> MALEGLRKKYKTRQELVKALTPKRRSIHLNSNGHSNGTPCSNADVLAHIKHFLSLAANSLEQHQQPISIVFQNKKKKGDTNSPDIHTTLDFPLNGPHLSTHQFKLKRCAILLNLLKVVMEKLPLGKNTTVRDIFYSNVELFQRQANVVQWLDVIRFNFKLSPRKSLNIIPAQKGLVYSPFPIDIYDNILTCENEPKMQKQTIFSGKPCLIPFFQDDAVIKLGTTSMCNIVIVEKEAVFTKLVNNYHKLSTNTMLITGKGFPDFLTRLFLKKLEQYCSNLISDCSIFTDADPYGISIALNYTHSNERNAYICTMANYKGIRITQVLAQNNEVHNKSIQLLSLNQRDYSLAKNLIASLTANSWDIATSPLKNVVIECQREIFFQKKAEMNEIDAGIFKYKSRHHHHHHHHHHGDYKDDDDKDYKDDDDKDYKDDDDK;> MARDITFLTVFLESCGAVNNDEAGKLLSAWTSTVRIEGPEPTDSNSLYIPLLPPGMLKIKLNFKMNDRLVTEEQELFTKLREIVGSSIRFWEEQLFYQVQDVSTIENHVILSLKCTILTDAQISTFISKPRELHTHAKGYPEIYYLSELSTTVNFFSKEGNYVEISHVIPHFNEYFSSLIVSQLEFEYPMVFSMISRLRLKWQQSSLAPISYALTSNSVLLPIMLNMIAQDKSSTTAYQILCRRRGPPIQNFQIFSIPAVTYNK;> MSKVFIATANAGKAHDADIFSVSACNSFTVSCSGDGYLKVWDNKLLDNENPKDKSYSHFVHKSGLHHVDVLQTIERDAFELCLVATTSFSGDLLFYRITREDETKKVIFEKLDLLDSDMKKHSFWALKWGASNDRLLSHRLVATDVKGTTYIWKFHPFADESNSLTLNWSPTLELQGTVESPMTPSQFATSVDISERGLIATGFNNGTVQISELSTLRPLYNFESQHSMINNSNSIRSVKFSPQGSLLAIAHDSNSFGCITLYETEFGERIGSLSVPTHSSQASLGEFAHSSWVMSLSFNDSGETLCSAGWDGKLRFWDVKTKERITTLNMHCDDIEIEEDILAVDEHGDSLAEPGVFDVKFLKKGWRSGMGADLNESLCCVCLDRSIRWFREAGGK;> MSIEEEDTNKITCTQDFLHQYFVTERVSIQFGLNNKTVKRINKDEFDKAVNCIMSWTNYPKPGLKRTASTYLLSNSFKKSATVSLPFILDDPVCMPKRVESNNNDTCLLYSDTLYDDPLIQRNDQAGDEIEDEFSFTLLRSEVNEIRPISSSSTAQILQSDYSALMYERQASNGSIFQFSSP

DNA double-strand breaks that initiate meiotic recombination are formed by the topoisomerase-relative enzyme Spo11, supported by conserved auxiliary factors. We report cryo-electron microscopy structures at up to 3.3-Å resolution of DNA-bound core complexes of Saccharomyces cerevisiae Spo11 with Rec102, Rec104 and Ski8. The core complex is monomeric (1:1:1:1 stoichiometry) and adopts a V shape with Spo11 at the base contacting the three other subunits. Spo11 is a central hub making extensive protein–protein and protein–DNA contacts.

We leveraged the tight binding to DNA ends to determine a cryo-EM structure of core complexes bound to a 23-bp hairpin DNA with a two-nucleotide 5′ overhang. Spo11 binds tightly to the free end of this substrate and with much lower affinity to the hairpin end. Core complexes were purified after expression in insect cells and incubated with Mg2+ and hairpin DNA. The structure of the protein–DNA complexes was solved at 3.7-Å resolution. The hairpin’s overhang end is anchored in a deep cleft between the Spo11 WH and Toprim domains. The remainder of the duplex makes non-sequence-specific contacts primarily with Spo11 and fewer with Rec102 and Rec104 but not with Ski8. We could trace the base, sugar and 5′-phosphate of the first nucleotide (A2) in the overhang adjacent to the terminal base pair. By contrast, the next overhang base (T1) could not be traced because of weak density. Residue Y135 involved in DNA covalent bond formation is on the opposite side of the DNA end from the Mg2+-coordinating E233, D288 and D290 residues.>GPSRATMALSRALRCCQRIFSWIPVIIISSVVLWSYYAYVFELCFVTLSNNLERVTYLLIFHVCFIMFCWTYWKAIFTPPSTPTKKFHLSYTDKERYEMEERPEVQKQILVDIAKKLPIFTRAQSGAIRFCDRCQVIKPDRCHHCSVCETCVLKMDHHSPWVNNCVGFSNYKFFLLFLSYSMIYCVFIASTVFQYFL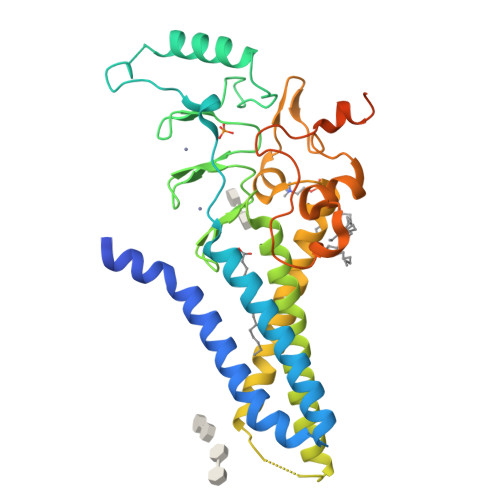KFWVGDLPNGPAKFHVLFLLFVALMFFVSLMFLFGYHCWLVAKNRSTLEAFSPPVFQNGPDRNGFNVGLSKNLRQVFGEHKKLWFIPVFTSQGDGHYFPLRTLRESENPLLANEEKWVEDGGSDEESADENGSSLLIRTESSNS[2x]> MLQVERPKLILDDGKRTDGRKPDELRSIKIELGVLKNADGSAIFEMGNTKAIAAVYGPKEMHPRHLSLPDRAVLRVRYHMTPFSTDERKNPAPSRREIELSKVIREALESAVLVELFPRTAIDVFTEILQADAGSRLVSLMAASLALADAGIPMRDLIAGVAVGKADGVIILDLNETEDMWGEADMPIAMMPSLNQVTLF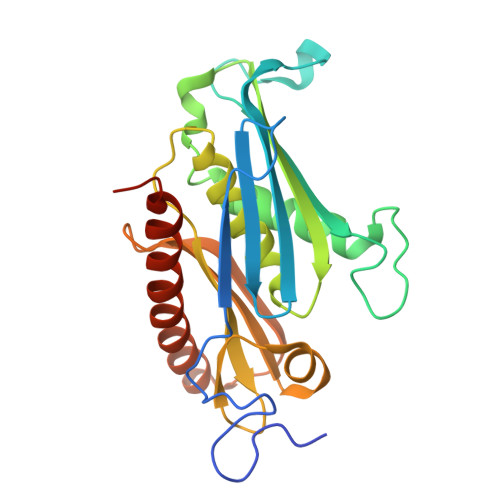QLNGSMTPDEFRQAFDLAVKGINIIYNLEREALKSKYVEFKEEGV2-(2-ETHOXYETHOXY)ETHANOL 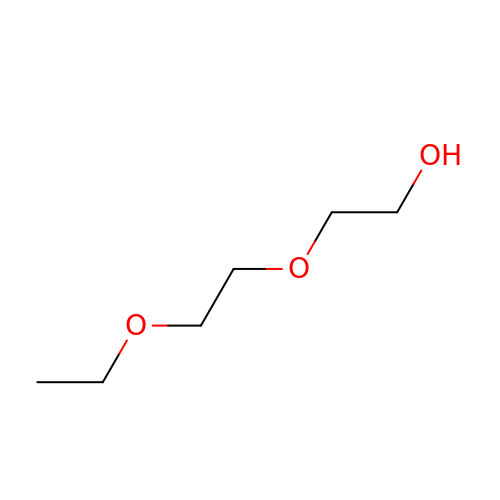| C6 H14 O3 | XXJWXESWEXIICW-UHFFFAOYSA-N>NLVQFGFMIECAIRNRRPALDFMNYGCYCGTVGRGTPVDDLDRCCQVHDECYATAEKHGCYPS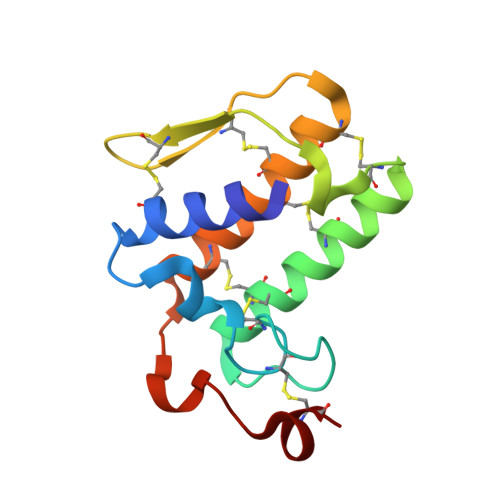LTTYQWECRQVGNECNSKTQCEVFVCACDLAAAKCLAQEDYNPAHFNINTGERCK[2x]>MAVPFVEDWDLVQTLGEGAYGEVQLAVNRVTEEAVAVKIVDMKRAVDCPENIKKEICINKMLNHENVVKFYGHRREGNIQYLFLEYCSGGELFDRIEPDIGMPEPDAQRFFHQLMAGVVYLHGIGITHRDIKPENLLLDERDNLKISDFGLATVFRYNNRERLLNKMCGTLPYVAPELLKRREFHAEPVDVWSCGIVLTAMLAGELPWDQPSDSCQEYSDWKEKKTYLNPWKKIDSAPLALLHKILVENPSARITIPDIKKDRWYNKPLKKG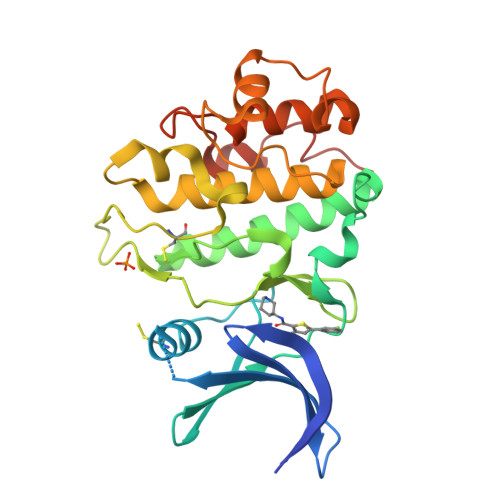AKRP[2x]>[2x]METLTVHAPSPSTNLPSYGNGAFSLSAPHVPGAGPLLVQVVYSFFQ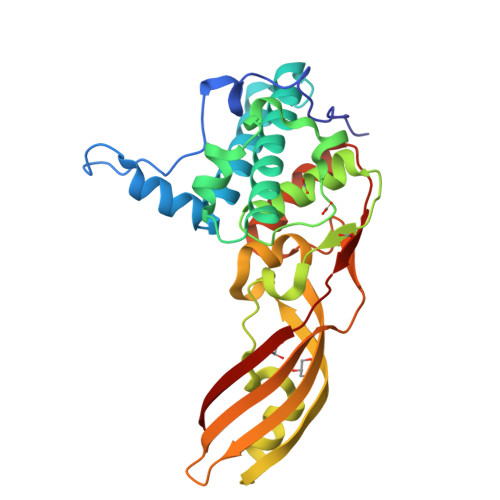SPNMCLQALTQLEDYIKKHGASNPLTLQIISTNIGYFCNADRNLVLHPGISVYDAYHFAKPAPSQYDYRSMNMKQMSGNVTTPIVALAHYLWGNGAERSVNIANIGLKISPMKINQIKDIIKSGVVGTFPVSTKFTHATGDYNVITGAYLGNITLKTEGTLTISANGSWTYNGVVRSYDDKYDFNASTHRGIIGESLTRLGAMFSGKEYQILLPGEIHIKESGKR> GSHMTCWLRGVTATFGRPAEWPGYLSHLCGRSAAMDLGPMRKSYRGDREAFEETHLTSLDPVKQFAAWFEEAVQCPDIGEANAMCLATCTRDGKPSARMLLLKGFGKDGFRFFTNFESRKGKELDSNPFASLVFYWEPLNRQVRVEGPVKKLPEEEAECYFHSRPKSSQIGAVVSHQSSVIPDREYLRKKNEELEQLYQDQEVPKPKSWGGYVLYPQVMEFWQGQTNRLHDRIVFRRGLPTGDSPLGPMTHRGEEDWLYERLAP

The enzyme pyridox(am)ine 5′‐phosphate oxidase (PNPO), whose catalytic action yields PLP, is one of the key players in this pathway. In humans, the different B6 vitamers, introduced with food, are interconverted through a salvage pathway which involves, besides kinases and phosphatases, the enzyme pyridoxine 5′‐phosphate (PNP)/pyridoxamine 5′‐phosphate (PMP) oxidase (PNPO) (di Salvo et al., 2011, 2012). This flavin mononucleotide (FMN)‐dependent enzyme, which produces PLP from PNP or PMP, plays an active role in vitamin B6 homeostasis. In both human and E. coli PNPO, PLP works as a regulator of its own production because it binds at an allosteric site of the enzyme, affecting the binding of substrate at the active site and inhibiting the catalytic activity (Barile et al., 2019, 2021). Mutations in the gene encoding PNPO are responsible for a severe form of neonatal epilepsy.

In order to further confirm the location of the PNPO allosteric site, we made several attempts to obtain the crystal structure of the protein‐PLP complex. On the basis of this previous experience, we carried out co‐crystallization attempts with either the wild type or the R225H variant of the human protein and PLP. We obtained crystals with both protein forms; however, PLP was detected only in the active site of the wild type protein, thus a clear indication about the location of the allosteric site was missing. A substantial part of the N‐terminal end is not visible in these structures: the electron density map starts from Glu46 in the R225H and from Ala47 in the wild type structure. Moreover, with respect to our structures, the conformation of the N‐terminal end in the previously published structure is different. The proteolytic cleavage of PNPO is not caused by the action of proteases during the purification, but it takes place in the bacterial cells, as evident from the western blot analysis of cell extracts. This observation indicates a marked flexibility of the N‐terminus, and could explain the fact that this region is missing in the electron density map of all the crystal structures solved so far. In the human PNPO, the coupling between the allosteric site and the active site is weaker, and PLP can bind simultaneously at the allosteric site and at the active site, forming a complex in which each subunit binds two PLP molecules. Although our x‐ray crystallography analyses were not successful in identifying the location of the PLP allosteric site, the results obtained with the site‐directed variants clearly show that the amino acid residues identified in the docking analysis are directly involved in the allosteric properties of the enzyme.Dexverapamil | 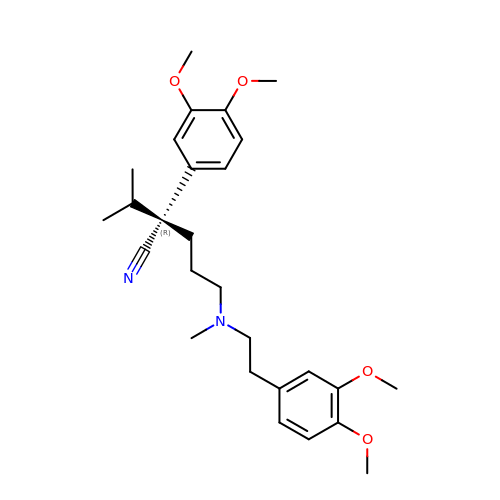C27 H38 N2 O4 | SGTNSNPWRIOYBX-HHHXNRCGSA-N>MVKEVVRTDSLKGRRGRLPSKPKSPQEPSPPSPPVSLISALVRAHVDSNPAMTSLDYSRFQANPDYQMSGDDTQHIQQFYDLLTGSMEIIRGWAEKIPGFADLPKADQDLLFESAFLELFVLRLAYRSNPVEGKLIFCNGVVLHRLQCVRGFGEWIDS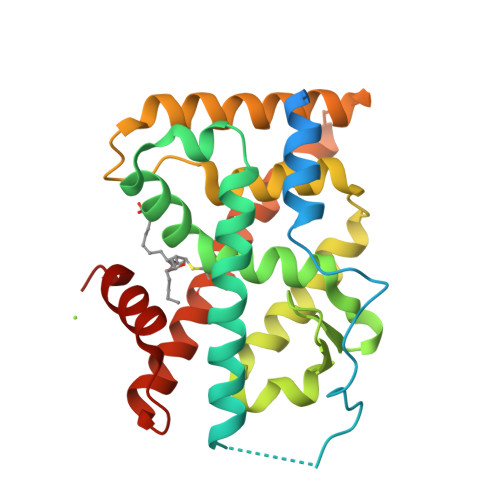IVEFSSNLQNMNIDISAFSCIAALAMVTERHGLKEPKRVEELQNKIVNCLKDHVTFNNGGLNRPNYLSKLLGKLPELRTLCTQGLQRIFYLKLEDLVPPPAIIDKLFLDTLPF[4x]> MQTTVTTMLLASVALAACAGGGSTPLPLPQQQPPQQEPPPPPVPLASRAACEALKDGNGDMVWPNAATVVEVAAWRDAAPATASAAALPEHCEVSGAIAKRTGIDGYPYEIKFRLRMPAEWNGRFFMEGGSGTNGSLSAATGSIGGGQIASALSRNFATIATDGGHDNAVNDNPDALGTVAFGLDPQARLDMGYNSYDQVTQAGKAAVARFYGRAADKSYFIGCSEGGREGMMLSQRFPSHYDGIVAGAPGYQLPKAGISGAWTTQSLAPAAVGLDAQGVPLINKSFSDADLHLLSQAILGTCDALDGLADGIVDNYRACQAAFDPATAANPANGQALQCVGAKTADCLSPVQVTAIKRAMAGPVNSAGTPLYNRWAWDAGMSGLSGTTYNQGWRSWWLGSFNSSANNAQRVSGFSARSWLVDFATPPEPMPMTQVAARMMKFDFDIDPLKIWATSGQFTQSSMDWHGATSTDLAAFRDRGGKMILYHGMSDAAFSALDTADYYERLGAAMPGAAGFARLFLVPGMNHCSGGPGTDRFDMLTPLVAWVERGEAPDQISAWSGTPGYFGVAARTRPLCPYPQIARYKGSGDINTEANFACAAPPLEHHHHHH

PETase cleaves BHET to MHET and EG, and the soluble MHET product is further hydrolyzed by MHETase to produce TPA and EG. Overall, the structure of MHETase is most similar to that of FAEs. The structural conservation between the hydrolase domains of MHETase and PETase is striking, and despite the large insertion of ∼240 residues representing the lid domain, residues Ser225, Asp492, and His528 effectively reconstitute the catalytic triad.

Of note, they pointed out the importance of Phe415 for substrate binding via an “induced fit” mechanism and highlighted Arg411 with respect to hydrogen bonding of the MHET carboxylate group, both of which are proposed to be drivers of substrate specificity. The only other amino acid with side-chain positioning correlated with ligand binding is Gln410. When Phe415 is in the open position, the side chain of Gln410 pivots toward the active site to a position wherein the heavy atoms would be as close as 1.8 Å to those of Phe415 if it were in the closed conformation. Given the observed dual occupancy for Phe415 positioning in the crystal structures, we simulated in triplicate (each simulation 150 ns in length) the four combinations of Phe415 position (open and closed) and active site occupancy (empty active site and MHET-bound). One of the MHETase disulfides is located at the active site, connecting cysteines (Cys224 and Cys529) adjacent to the catalytic residues (Ser225 and His528, respectively), which is conserved in tannase family members. A similar Ca2+ binding site was characterized for Aspergillus oryzae FaeB (AoFaeB), wherein it was hypothesized to have a role in stabilizing the lid domain.> TQAEKTATDLPPGFSGKAGSVNATPGTKGLDGPTPLADGSFDATIFGPAKELKSADDILNVHRRNAKDPFAVGAVDAPLVITEFSDFECPFCA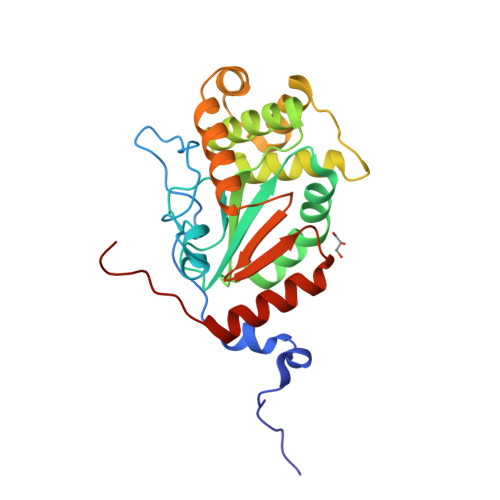RWSNQTEPTLMEEYVSKGLVRIEWNDLPVNGEHALAAAKAGRAAAAQGKFDEFRKALFEASRNVSGHPNNTLKDFERFARNAGVKDMERFSREAQDSTYDEVLAKAADYAHGLGVSGTPAFVVGTQYISGAQPTEEFIKVIESELKKSPTFSTPSSH>[3x]MIGFLTDWGLKSHYVGVAKAVIKRINPSAEIIDITHEVEPFNVRKASHVLYRASLDFPPSTVFLVVVDYGVGTSRKAIVMKTKNDQYFVAPDNGVLTVVAEEYGVAEIREIENRELFYKKNPSFTFHGRDIF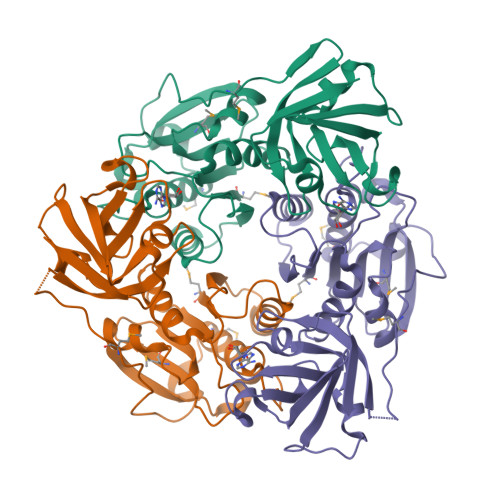APVAAHLDMGLPLERVGDRLLSYEVLKMRKPVVENEKVIGEVAIVDTFGNVSTNIPFDLFLKLSVDFDDVVRVRVGRKEFKAAVAKAFGDVDTGELLVHPDSAGFLEIAVNLGDASQVLSVKEGDEIEICR> RRTSRRKRAKV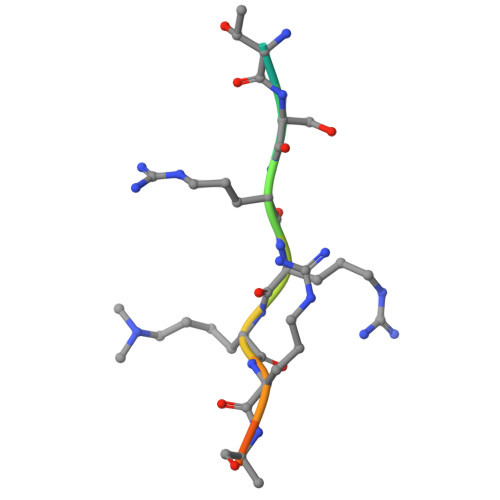E[4-(imidazo[4,5-d]pyrrolo[2,3-b]pyridin-1(6H)-yl)piperidin-1-yl][(2S)-1-(propan-2-yl)pyrrolidin-2-yl]methanone | C21 H28 N6 O | 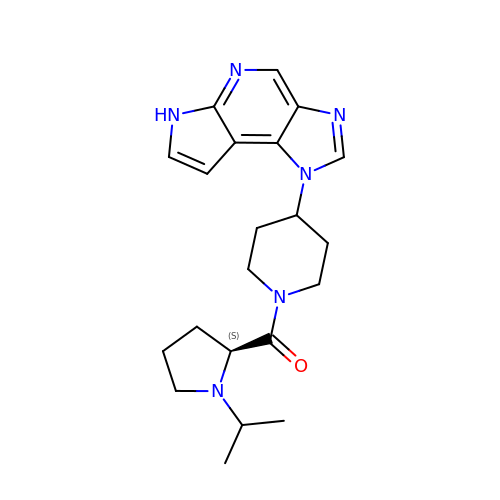XDHQVHVOFHWRNB-SFHVURJKSA-N> NYCNQMMKSRNLTKDR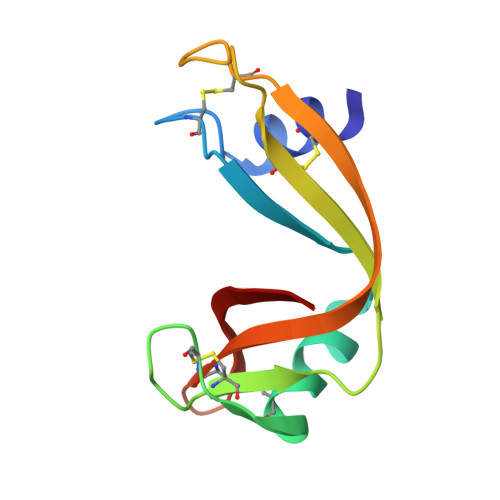CKPVNTFVHESLADVQAVCSQKNVACKNGQTNCYQSYSTMSITDCRETGSSKYPNCAYKTTQANKHIIVACEGNPYVPVHFDASV> LVPRGSHMNTSELRICRINKESGPCTGGEELFLLCDKVQKEDISVVFSTASWEGRADFSQADVHRQFAIVFKTPPYEDLEISEPV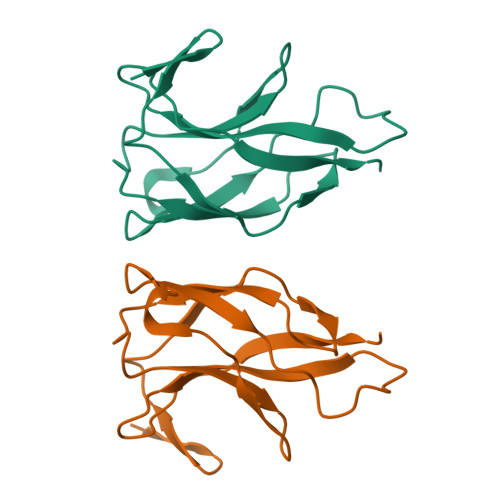TVNVFLQRLTDGVCSEPLPFTYLPR> MIPIKVSMRNLSSLTIAGGSTISSIDIPLNPLGVPPSTIKGTMRTAVHNLLPNGYTSCGEVEPESIREAHKNGVCDVCKLFGYPDSLTGCFTIDVSKTDYRTSYITRVSIDDKTQRAKEGSLFTQQIILPNSDISFTVYYNCND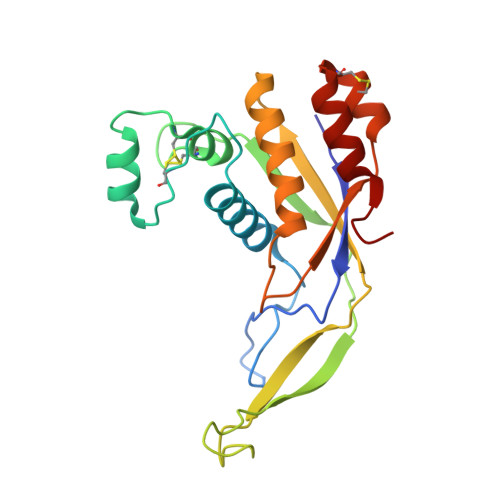ERLFKLLLYSILDLRYWRLGRNTMIDVKVNNVEEICKSVKCDEEINGILNQLSRYLWE>MVVIGEKFPEVEVKTTHGVIKLPDYFTKQGKWFILFSHPADFTPVCTTEFYGMQKRVEEFRKLGVEPIGLSVDQVFSHIKWIEWIKDNLSVEIDFPVIADDRGELAEKLGMIPSGATITARAVFVVDDKGIIRAIVYYPAEVGRDWDEILRLVKALKISTEKGVALPHKWPNNELIGDKVIVPPASTIE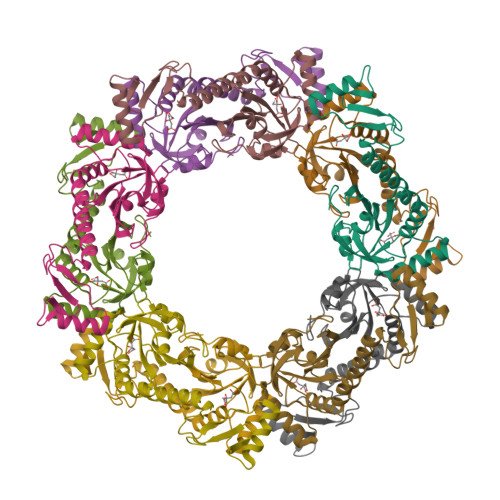EKKQREEAKAKGEIECYDWWFCYKKLE[20x]> MKVFKAVIGAIL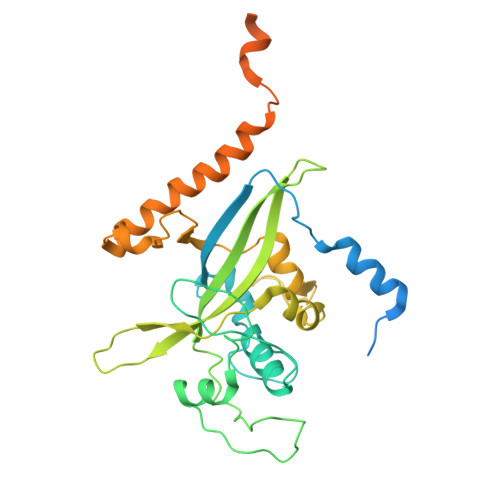AATVSIPSVAQENTNNRSPQVGRAPRNTEVEQMTTLSNRAQEFNRRLTQKTDNAPWRRVVYRRVDLMEESNAVLYYPPRPIGDRKNLFSTIFGLINSNSLDVYEYLDGFEAFTDQYKIKFQEFLDRFGIYYQPSTNKNAELFKVADSDIPSAEVKAYYVKEEWYFTPTNSDVDIKIQAICPIMTGQDEFGEVRNQPLFWIPYENIRPYIARERVMLSSLNNTRNSTIDDFFRLNLYKGDIVKTENLHNRALAEYCPTPDSMKMESKRIDKELQGFRDGLFVTQDTTWMKQVETKKSKGKKLEKARGKNITSRTRGQGEGAAETEAVEPKKQKASKNKAATRSVRRRK> MRGSFANDATFEIKKCDLHRLEEGPPVTTVLTREDGLKYYRMMQTVRRMELKADQLYKQKIIRGFCHLCDGQEACCVGLEAGINPTDHLITAYRAHGFTFTRGLSVREILAELTGRKGGCAKGKGGSMHMYAKNFYGGNGIVGAQV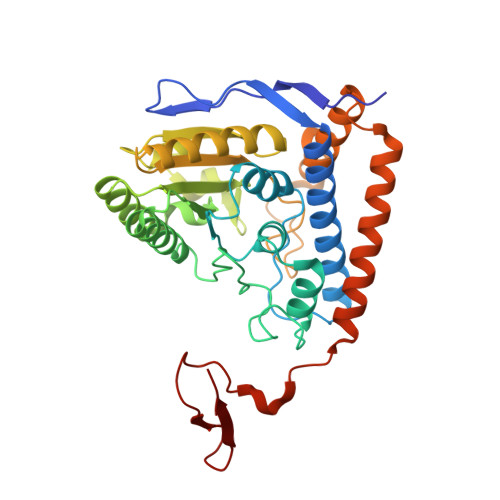PLGAGIALACKYNGKDEVCLTLYGDGAANQGQIFEAYNMAALWKLPCIFICENNRYGMGTSVERAAASTDYYKRGDFIPGLRVDGMDILCVREATRFAAAYCRSGKGPILMELQTYRYHGHEMSDPGVSYRTREEIQEVRSKSDPIMLLKDRMVNSNLASVEELKEIDVEVRKEIEDAAQFATADPEPPLEELGYHIYSSDPPFEVRGANQWIKFKSVS> GSHMTKELRIVNGSFTVKKVLNNNVLIASHHKYSEVVLIGKGIGFGKKQDDVIEDKGYDKMFILKDEKEQKQFKKLLDYVDEKLVDISNDVIYHISNRTNHSLNEHIHIALTDHIAFAIKRQQQG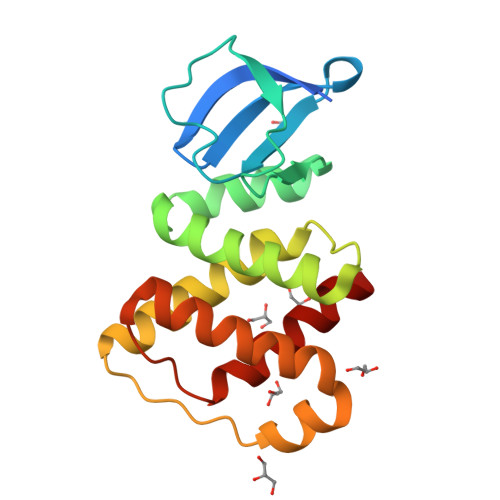FDMKNPFLMETQSLYPEEYQIAKEVIDMINEKAGLCLPEGEIGFIALHIHSALTN Stem-loop 5 (SL5, residues 150 to 294) contains the start codon of open reading frame 1a/b (ORF1a/b, residues 266 to 268). Additionally, phylogenetic covariance analysis and chemical probing experiments have shown that SL5′s secondary structure forms a four-way junction that sequesters the genome’s start codon within one of its helical stems. Beyond SARS-CoV-2, the multi-way junction and the sequestration of the start codon in a stem are conserved features across most coronaviruses, despite large sequence divergence from SARS-CoV-2 (average sequence identity of 51% for the NCBI Reference Sequences for alpha- and betacoronaviruses). SL5 has been proposed to play a role in protein–RNA or RNA–RNA binding because of its conserved hexaloops, characterized by 5′-UUYYGU-3′ (Y = C, U) repeat loop motifs.

Cryo-EM image reconstruction of the SARS-CoV-2 SL5 domain (residues 159 to 282, 124 nt, 40.0 kDa) shows a single, well-defined 3D structure resolved to 4.7 Å resolution. Four helices extend from one junction, all with clear major and minor grooves. The approximate lengths of these helices align with the expected lengths of the stems in the M2-seq secondary structure, enabling the unambiguous identification of SL5c as the shortest stem and SL5b as the medium-length stem. The junction is well resolved, revealing two pairs of coaxially stacked helices and a hole at the junction that clearly demarcates the backbone connectivity between helical pairs. This connectivity also enables the unambiguous assignment of SL5a and the SL5-stem into the map. Auto-DRRAFTER converged on a T-shaped conformation wherein the SL5-stem forms the “leg” of the T-shape, SL5a and SL5b stack end-to-end to form the perpendicular “arms” of the T-shape, and SL5c juts out of the plane of the T-shape at the junction. The UUYYGU hexaloops of SL5a and SL5b are positioned at the “hands” of the T-shape, positioned 84.2 ± 0.8 Å away from each other (N = 30). The two pairs of coaxially stacked helices, SL5a:SL5b and SL5-stem:SL5c have an inter-helical angle of 84.3 ± 0.5° but do not form any significant tertiary interactions (N = 30). The four-way junction is well converged and has atomic resolvability above what is expected at 4.7 Å resolution (0.41 Q-score for junction atoms on average, with an expected 0.35 Q-score at that resolution). Based on our cryo-EM analysis, the SL5 domain of SARS-CoV-2 has a defined tertiary fold, as opposed to a highly flexible ensemble.

> GGACACGAGUAACUCGUCUAUCUUCUGCAGGCUGCUUACGGUUUCGUCCGUGUUGCAGCCGAUCAUCAGCACAUCUAGGUUUCGUCCGGGUGUGACCGAAAGGUAAGAUGGAGAGCCUUGUCCC>[2x]SGNRGVVYLGSGKVEVQKIDYPKMQDPRGKKIEHGVILKVVSTNICGSDQHMVRGRTTAQVGLVLGHEITGEVIEKGRDVENLQIGDLVSVPFNVACGRCRSCKEM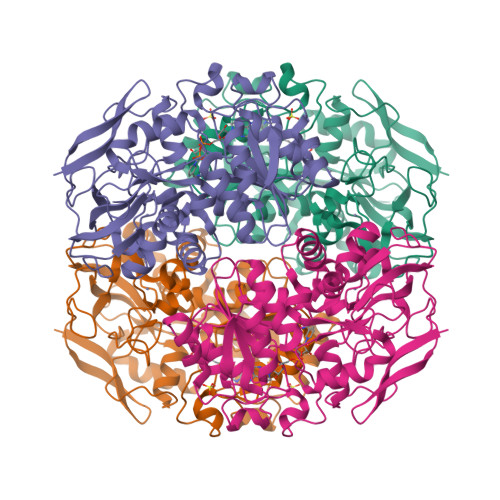HTGVCLTVNPARAGGAYGYVDMGDWTGGQAEYVLVPYADFNLLKLPDRDKAMEKIRDLTCLSDILPTGYHGAVTAGVGPGSTVYVAGAGPVGLAAAASARLLGAAVVIVGDLNPARLAHAKAQGFEIADLSLDTPLHEQIAALLGEPEVDCAVDAVGFEARGHGHEGAKHEAPATVLNSLMQVTRVAGKIGIPGLYVTEDPGAVDAAAKIGSLSIRFGLGWAKSHSFHTGQTPVMKYNRALMQAIMWDRINIAEVVGVQVISLDDAPRGYGEFDAGVPKKFVIDPHKTFSAA>[2x]MVDLKRLRQEPEVFHRAIREKGVALDLE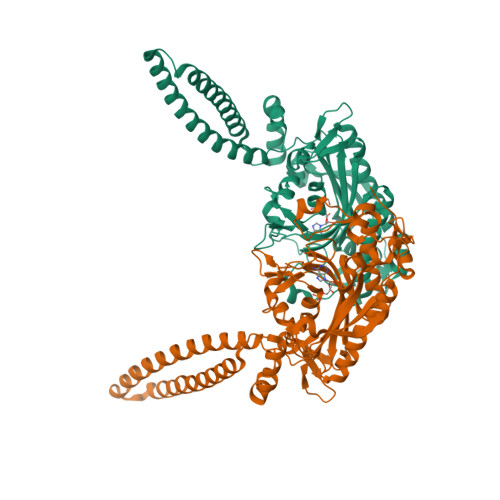ALLALDREVQELKKRLQEVQTERNQVAKRVPKAPPEEKEALIARGKALGEEAKRLEEALREKEARLEALLLQVPLPPWPGAPVGGEEANREIKRVGGPPEFSFPPLDHVALMEKNGWWEPRISQVSGSRSYALKGDLALYELALLRFAMDFMARRGFLPMTLPSYAREKAFLGTGHFPAYRDQVWAIAETDLYLTGTAEVVLNALHSGEILPYEALPLRYAGYAPAFRSEAGSFGKDVRGLMRVHQFHKVEQYVLTEASLEASDRAFQELLENAEEILRLLELPYRLVEVATGDMGPGKWRQVDIEVYLPSEGRYRETHSCSALLDWQARRANLRYRDPEGRVRYAYTLNNTALATPRILAMLLENHQLQDGRVRVPQALIPYMGKEVLEPCG> MVEATAQETDRPRFSFSIAAREGKARTGTIEMKRGVIRTPAFMPVGTAATVKALKPETVRATGADIILGNTYHLMLRPGAERIAKLGGLHSFMGWDRPILTDSGGFQVMSLSSLTKQSEEGVTFKSHLDGSRHMLSPERSIEIQHL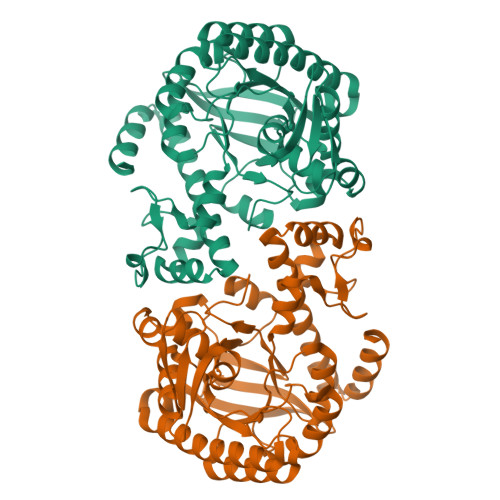LGSDIVMAFDECTPYPATPSRAASSMERSMRWAKRSRDAFDSRKEQAENAALFGIQQGSVFENLRQQSADALAEIGFDGYAVGGLAVGEGQDEMFRVLDFSVPMLPDDKPHYLMGVGKPDDIVGAVERGIDMFDCVLPTRSGRNGQAFTWDGPINIRNARFSEDLKPLDSECHCAVCQKWSRAYIHHLIRAGEILGAMLMTEHNIAFYQQLMQKIRDSISEGRFSQFAQDFRARYFARNS> AGRKVVVVGGGTGGATAAKYIKLADPSIEVTLIEPNETYYTCYMSNEVIGGDRELASLRVGYDGLRAHGIQVVHDSALGIDPDKKLVKTAGGAEFAYDRCVVAPGIDLLYDKIEGYSEALAAKLPHAWKAGEQTALLRRQLESMDDGGVVIIAPPAPPFRCPPGPYERASQIAHYLKAHKSKSKVIILDNSQTFSKQAQFTKGWERLYGFGTENALIEWHPGPDAAVVKTDTEAMTVETSFGETFKAAVINLIPPQRAGKIAQSASLTNDSGWCPVDIRTFESSLQPGIHVIGDACNAAPMPKSAYSANSQAKVAAAAVVALLKGEEPGTPSYLNTCYSILA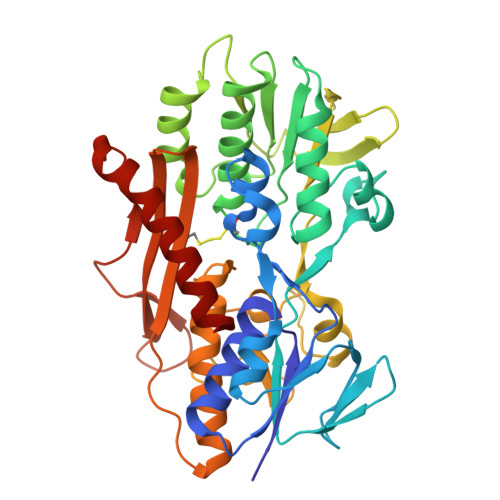PGYGISIAAVYRPNAEGKAIEAVPDSGGITPVDAPDWVLEREVQYAHSWYNNIVHDTFG Transcriptional co-regulators of the SRO group are characterized by a conserved PARP domain and a C-terminal RST (RCD1 SRO TAF4) domain that binds transcription factors. Although the PARP domain in SRO proteins is strictly conserved, residues of the His–Tyr–Glu triad deviate from the consensus sequence in SRO proteins. Liu et al. (2014) proposed that the bread wheat (T. aestivum) Ta-SRO1 protein can catalyze poly-ADP-ribosylation reactions although the His–Tyr–Glu is replaced by Leu–His–His in this protein. We present a structural analysis of the Ta-sro1 PARP domain at 2.1 Å resolution together with in vitro and in vivo assays of biochemical function, providing strong evidence that Ta-sro1 is unlikely to have PARP activity.

The domain adopts the typical PARP fold with a β–α–loop–β–α signature at the donor site that binds NAD+. The donor site loop (D-loop) occludes the proposed active site of Ta-sro1 and is only partially resolved in the structure with little interpretable electron density for amino acids Met334–Gly336. The structure confirms that the His–Tyr–Glu triad is not conserved in Ta-sro1. The position of the conserved His residue is taken by Ta-sro1 Leu312. The Tyr that stacks with the nicotinamide ribose ring in canonical PARP enzymes is replaced by His344 in Ta-sro1. The catalytic Glu that is specifically required for the PAR chain elongating polymerase activity of PARPs is replaced by Ta-sro1 His407. Thr343 (Ala in Ta-SRO1) is located close to the proposed active site and its side chain is positioned toward the hydrophobic core of the protein formed by residues Leu345, Val330, Leu328, Ile419, Val415, and Ile410. However, our Ta-sro1 PARP domain crystal structure reveals that the Ta-sro1 Thr343 side chain points in the opposite direction and toward a hydrophobic area forming the basis of the postulated NAD+-binding site. The second polymorphic amino acid, Val250 (Gly in Ta-SRO1) is positioned on the opposite side of the domain and located close to the N-terminus of the crystallized construct.

>GPIGQPVDSAVRKLLLEGAGQPFSEENIIGIYRTPLVDQQGRARFNLFQKELEATKMHRGNANVRYAWLPCSKDTMEEMMMRGVLEVTKPMLGPVYGIGTHLAPANCAQTCASYSDIDENGIMRMMLCRVIMGNVEVVLPGSKQFQPTNERFDSGVDDLQKPKHYIIWDANVHRHIYAEYAVVIKAPSMTN[2x]> DDLPYRFGLGKADITGEAAEVGMMGYSSLEQKTAGIHMRQWARAFVIEEAASGRRLVYVNTDLGMIFQAVHLKVLARLKAKYPGVYDENNVMLAATHTHSGPGGFSHYAMYNLSVLGFQEKTFNAIVDGIVRSIERAQARLQPGRLFYGSGELRNASRNRSLLSHLKNPDIAGYEDGIDPQMSVLSFVDANGELAGAISWF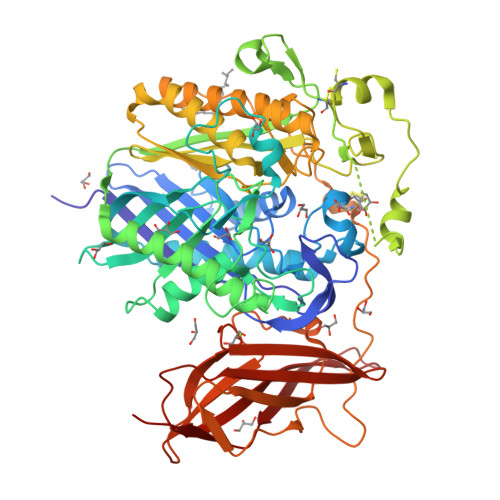PVHSTSMTNANHLISPDNKGYASYHWEHDVSRKSGFVAAFAQTNAGNLSPNLNLKPGSGPFDNEFDNTREIGLRQFAKAYEIAGQAQEEVLGELDSRFRFVDFTRLPIRPEFTDGQPRQLCTAAIGTSLAAGSTEDGPGPLGLEEGNNPFLSALGGLLTGVPPQELVQCQAEKTILADTGNKKPYPWTPTVLPIQMFRIGQLELLGAPAEFTVMAGVRIRRAVQAASEAAGIRHVVFNGYANAYASYVTTREEYAAQEYEGGSTLYGPWTQAAYQQLFVDMAVALRERLPVETSAIAPDLSCCQMNFQTGVVADDPYIGKSFGDVLQQPRESYRIGDKVTVAFVTGHPKNDLRTEKTFLEVVNIGKDGKQTPVTVATDNDWDTQYRWERVGISASKATISWSIPPGTEPGHYYIRHYGNAKNFWTQKISEIGGSTRSFEVLGTTP>[2x]MASMTGGQQMGRGSSTSLYKKAGLMPSPMEDIEEILITEEQLKAKVKELGEMITRDYEGKDLVLIGVLKGAIMFMSGLSRAIDLPLSIDFLAVSSYGSSTKSSG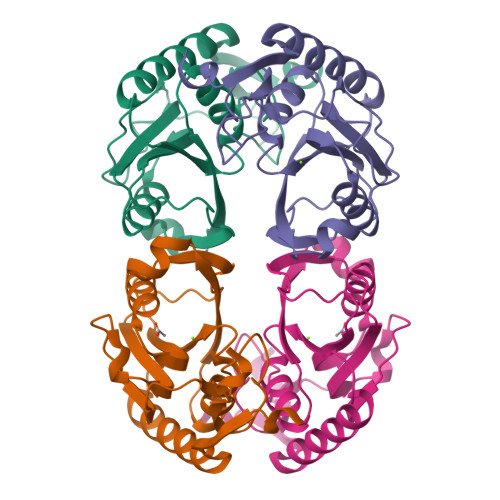IVKIIKDHDIDIEGKDVLIVEDIIDSGLTLAYLRETLLGRKPRSLKICTILDKPERREADVKVDYCGFKIPDKFVVGYGLDYAEKYRNLPFIGVLKPELYK N-(CARBOXYMETHYL)-N,N-DIMETHYL-3-[(1-OXODODECYL)AMINO]-1-PROPANAMINIUM INNER SALT | C19 H38 N2 O3 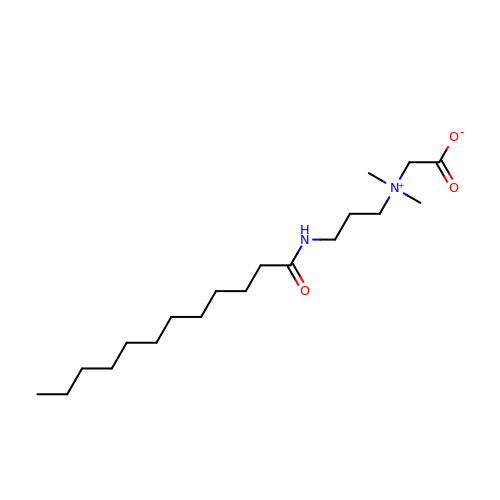| MRUAUOIMASANKQ-UHFFFAOYSA-N> XXXXXXXXXXXXXXXXXXXXXXXXXXXXXXXXXXXXXXXXXXXXXXXXXXXXXXXXXXXXXXXXXXXXXXXXXXXXXXXXXXXXXXXXXXXXXXXXXXXXXXXXXXXXXXXXXXXXXXXXXXXXXXXXXXXXXXXXXXXXXXXXXXXXXXXXXXXXXXXXXXXXXXXXXXXXXXXXXXXXXXXXXXXXXXXXXXXXXXXXXXXXXXXXXXXXXXXXXXXXXXXXXXXXXXXXXXXXXXXXXXXXXXXXXXXXXXXXXXXXXXXXXXXXXXXXXXXXXXXXXXXXXXXXXXXXXXXXXXXXXXXXXXFSTNFRDTVDILVGWHIDHTQKPSLTQQVSGWLQSLEPFWVADLAFSTTLLGQFLEDMEAYAEDLSHVASGESVDEDVPPPSVSLPKLAALLRVFSTVVRSIGERFSPIRGPPITEAYVTDVLYRVMRCVTAANQVFFSEAVLTAANECVGVLLGSLDPSMTIHCDMVITYGLDQLENCQTCGTDYIISVLNLLTLIVEQINTKLPSSFVEKLFIPSSKLLFLRYHKEKEVVAVAHAVYQAVLSLKNIPVLETAYKLILGEMTCALNNLLHSLQLPEACSEIKHEAFKNHVFNVDNAKFVVIFDLSALTTIGNAKNSLIGMWALSPTVFALLSKNLMIVHSDLAVHFPAIQYAVLYTLYSHCTRHDHFISSSLSSSSPSLFDGAVISTVTTATKKHFSIILNLLGILLKKDNLNQDTRKLLMTWALEAAVLMRKSETYAPLFSLPSFHKFCKGLLANTLVEDVNICLQACSSLHALSSSLPDDLLQRCVDVCRVQLVHSGTRIRQAFGKLLKSIPLDVVLSNNNHTEIQEISLALRSHMSKAPSNTFHPQDFSDVISFILYGNSHRTGKDNWLERLFYSCQRLDKRDQSTIPRNLLKTDAVLWQWAIWEAAQFTVLSKLRTPLGRAQDTFQTIEGIIRSLAAHTLNPDQDVSQWTTADNDEGHGNNQLRLVLLLQYLENLEKLMYNAYEGCANALTSPPKVIRTFFYTNRQTCQDWLTRIRLSIMRVGLLAGQPAVTVRHGFDLLTEMKTTSLSQGNELEVTIMMVVEALCELHCPEAIQGIAVWSSSIVGKNLLWINSVAQQAEGRFEKASVEYQEHLCAMTGVDCCISSFDKSVLTLANAGRNSASPKHSLNGESRKTVLSKPTDSSPEVINYLGNKACECYISIADWAAVQEWQNSIHDLKKSTSSTSLNLKADFNYIKSLSSFESGKFVECTEQLELLPGENINLLAGGSKEKIDMKKLLPNMLSPDPRELQKSIEVQLLRSSVCLATALNPIEQDQKWQSITENVVKYLKQTSRIAIGPLRLSTLTVSQSLPVLSTLQLYCSSALENTVSNRLSTEDCLIPLFSEALRSCKQHDVRPWMQALRYTMYQNQLLEKIKEQTVPIRSHLMELGLTAAKFARKRGNVSLATRLLAQCSEVQLGKTTTAQDLVQHFKKLSTQGQVDEKWGPELDIEKTKLLYTAGQSTHAMEMLSSCAISFCKSVKAEYAVAKSILTLAKWIQAEWKEISGQLKQVYRAQHQQNFTGLSTLSKNILTLIELPSVNTMEEEYPRIESESTVHIGVGEPDFILGQLYHLSSVQAPEVAKSWAALASWAYRWGRKVVDNASXXXXXXXXXXXXXXXXXXXXXXXXXXXXXXXXXXXXXXXXXXXXXXXXXXXXXXXXXXXXXXXXXXXXXXXXXXXXXXXXXXXXXXXXEGVIKVWRKVVDRIFSLYKLSCSAYFTFLKLNAGQIPLDEDDPRLHLSHRVEQSTDDMIVMATLRLLRLLVKHAGELRQYLEHGLETTPTAPWRGIIPQLFSRLNHPEVYVRQSICNLLCRVAQDSPHLILYPAIVGTISLSSESQASGNKFSTAIPTLLGNIQGEELLVSECEGGSPPASQDSNKDEPKSGLNEDQAMMQDCYSKIVDKLSSANPTMVLQVQMLVAELRRVTVLWDELWLGVLLQQHMYVLXXXXXXXXXXXXXXXXXXXXXXXXXXXXXXXXXXXXXXXXXXXXXXXXXXXXXXXXPHEKWFQDNYGDAIENALEKLKXXXXXXXXXXXXXXXXXXXXXXXXXXXXXXXYILRLEEISPWLAAMTNTEIALPGEVSARDTVTIHSVGGTITILPTKTKPKKLLFLGSDGKSYPYLFKGLEDLHLDERIMQFLSIVNTMFATINRQETPRFHARHYSVTPLGTRSGLIQWVDGATPLFGLYKRWQQREAALQAQKAQDSYQTPQNPGIVPRPSELYYSKIGPALKTVGLSLDVSRRDWPLHVMKAVLEELMEATPPNLLAKELWSSCTTPDEWWRVTQSYARSTAVMSMVGYIIGLGDRHLDNVLIDMTTGEVVHIDYNVCFEKGKSLRVPEKVPFRMTQNIETALGVTGVEGVFRLSCEQVLHIMRRGRETLLTLLEAFVYDPLVDWTAGGEAGFAGAVYGGGGQQAESKQSKREMEREITRSLFSSRVAEIKVNWFKNRDEMLVVLPKLDGSLDEYLSLQEQLTDVEKLQGKLLEEIEFLEGAEGVDHPSHTLQHRYSEHTQLQTQQRAVQEAIQVKLNEFEQWITHYQAAFNNLEATQLASLLQEISTQMDLGPPSYVPATAFLQNAGQAHLISQCEQLEGEVGALLQQRRSVLRGCLEQLHHYATVALQYPKAIFQKHRIEQWKTWMEELICNTTVERCQELYRKYEMQYAPQPPPTVCQFITATEMTLQRYAADINSRLIRQVERLKQEAVTVPVCEDQLKEIERCIKVFLHENGEEGSLSLASVIISALCTLTRRNLMMEGAASSAGEQLVDLTSRDGAWFLEELCSMSGNVTCLVQLLKQCHLVPQDLDIPNPMEASETVHLANGVYTSLQELNSNFRQIIFPEALRCLMKGEYTLESMLHELDGLIEQTTDGVPLQTLVESLQAYLRNAAMGLEEETHAHYIDVARLLHAQYGELIQPRNGSVDETPKMSAGQMLLVAFDGMFAQVETAFSLLVEKLNKMEIPIAWRKIDIIREARSTQVNFFDDDNHRQVLEEIFFLKRLQTIKEFFRLCGTFSKTLSGSSSLEDQNTVNGPVQIVNVKTLFRNSCFSEDQMAKPIKAFTADFVRQLLIGLPNQALGLTLCSFISALGVDIIAQVEAKDFGAESKVSVDDLCKKAVEHNIQIGKFSQLVMNRATVLASSYDTAWKKHDLVRRLETSISSCKTSLQRVQLHIAMFQWQHEDLLINRPQAMSVTPPPRSAILTSMKKKLHTLSQIETSIATVQEKLAALESSIEQRLKWAGGANPALAPVLQDFEATIAERRNLVLKESQRASQVTFLCSNIIHFESLRTRTAEALNLDAALFELIKRCQQMCSFASQFNSSVSELELRLLQRVDTGLEHPIGSSEWLLSAHKQLTQDMSTQRAIQTEKE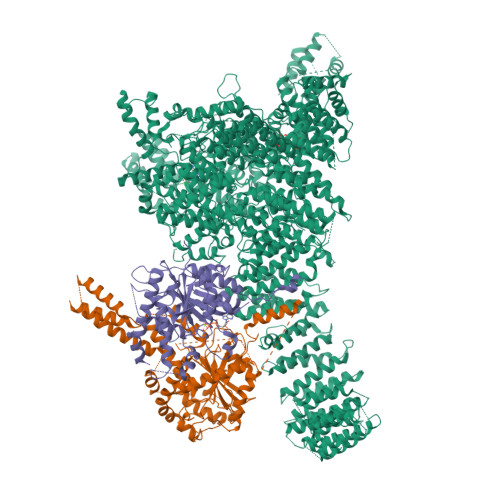QQIETVCETIQNLVDNIKTVLTGHNRQLGDVKHLLKAMAKDEEAALADGEDVPYENSVRQFLGEYKSWQDNIQTVLFTLVQAMGQVRSQEHVEMLQEITPTLKELKTQSQSIYNNLVSFASPLVTDATNECSSPTSSATYQPSFAAAVRSNTGQKTQPDVMSQNARKLIQKNLATSADTPPSTVPGTGKSVACSPKKAVRDPKTGKAVQERNSYAVSVWKRVKAKLEGRDVDPNRRMSVAEQVDYVIKEATNLDNLAQLYEGWTAWV;> MAGPVSLRDLLMGASAWMGSESPGGSPTEGGGSAAGGPEPPWREDEICVVGIFGKTALRLNSEKFSLVNTVCDRQVFPLFRHQDPGDPGPGIRTEAGAVGEAGGAEDPGAAAGGSVRGSGAVAEGNRTEAGSQDYSLLQAYYSQESKVLYLLLTSICDNSQLLRACRALQSGEAGGGLSLPHAEAHEFWKHQEKLQCLSLLYLFSVCHILLLVHPTCSFDITYDRVFRALDGLRQKVLPLLKTAIKDCPVGKDWKLNCRPCPPRLLFLFQLNGALKVEPPRNQDPAHPDKPKKHSPKRRLQHALEDQIYRIFRKSRVLTNQSINCLFTVPANQAFVYIVPGSQEEDPVGMLLDQLRSHCTVKDPESLLVPAPLSGPRRYQVMRQHSRQQLSFHIDSSSSSSSGQLVDFTLREFLWQHVELVLSKKGFDDSVGRNPQPSHFELPTYQKWISAASKLYEVAIDGKEEDLGSPTGELTSKILSSIKVLEGFLDIDTKFSENRCQKALPMAHSAYQSNLPHNYTMTVHKNQLAQALRVYSQHARGPAFHKYAMQLHEDCYKFWSNGHQLCEERSLTDQHCVHKFHSLPKSGEKPEADRNPPVLYHNSRARSTGACNCGRKQAPRDDPFDIKAANYDFYQLLEEKCCGKLDHINFPVFEPSTPDPAPAKNESSPAPPDSDADKLKEKEPQTQGESTSLSLALSLGQSTDSLGTYPADPQAGGDNPEVHGQVEVKTEKRPNFVDRQASTVEYLPGMLHSNCPKGLLPKFSSWSLVKLGPAKSYNFHTGLDQQGFIPGTNYLMPWDIVIRTRAEDEGDLDTNSWPAPNKAIPGKRSAVVMGRGRRRDDIARAFVGFEYEDSRGRRFMCSGPDKVMKVMGSGPKESALKALNSDMPLYILSSSQGRGLKPHYAQLMRLFVVVPDAPLQIILMPQVQPGPPPCPVFYPEKQEITLPPDGLWVLRFPYAYVTERGPCFPPKENVQLMSYKVLRGVLKAVTQ;> MSESGHSQPGLYGIERRRRWKEPGSGGPQNLSGPGGRERDYIAPWERERRDASEETSTSVMQKTPIILSKPPAERSKQPPPPTAPAAPPAPAPLEKPIVLMKPREEGKGPVAVTGASTPEGTAPPPPAAPAPPKGEKEGQRPTQPVYQIQNRGMGTAAPAAMDPVVGQAKLLPPERMKHSIKLVDDQMNWCDSAIEYLLDQTDVLVVGVLGLQGTGKSMVMSLLSANTPEEDQRTYVFRAQSAEMKERGGNQTSGIDFFITQERIVFLDTQPILSPSILDHLINNDRKLPPEYNLPHTYVEMQSLQIAAFLFTVCHVVIVVQDWFTDLSLYRFLQTAEMVKPSTPSPSHESSSSSGSDEGTEYYPHLVFLQNKARREDFCPRKLRQMHLMIDQLMAHSHLRYKGTLSMLQCNVFPGLPPDFLDSEVNLFLVPFMDSEAESENPPRAGPGSSPLFSLLPGYRGHPSFQSLVSKLRSQVMSMARPQLSHTILTEKNWFHYAARIWDGVRKSSALAEYSRLLA WXG100 proteins are a group of proteins of approximately ∼100 residues in length that contain a conserved “Trp-Xaa-Gly (WXG)” motif. To investigate how specific sequence motifs translate into specific structural features, we determined the atomic structures of two representative complexes, the heterodimeric CFP-10/ESAT-6 complex and the homodimeric sagEsxA assembly. The overall structures of the two protein complexes are similar, with both forming a four-helix bundle, in which each monomer consists of a helix-loop-helix structural motif. However, the novelty of this contribution is that by using the iterative bio-informatics approach, we can show that the WXG100 protein superfamily can be divided into three subfamilies: CFP-10-, ESAT-6- and sagEsxA-like.

The sagEsxA-like proteins form a homodimer and the structure of the sagEsxA shows that the driving force for the interdimer interactions is principally hydrophobic in nature. At the inter-dimeric interface, hydrophobic residues are prevalent in sagEsxA-like proteins although there is a pair of hydrophilic residues Y18 and Q36 within the hydrophobic core of sagEsxA. The side chains of these residues form hydrogen bonds within the hydrophobic core of the four-helix-bundle complex (inset) and the presence of these hydrogen bond pairs between Y18 and Q36 is indicative of the anti-parallel homodimer arrangement found in the sagEsxA subfamily of WXG100 proteins. As a result, this conserved pair of mutations can be seen as a fingerprint of anti-parallel homodimeric WXG100 proteins. In addition, it contains a 310-helix with hydrogen bonds originating only from main chain atoms, whereas, the loop of sagEsxA (residues 43–48) consists only of a single tight β-turn. The CFP-10 subfamily is structurally more closely related to the sagEsxA than to the ESAT-6 subfamily. This is reflected by a root mean square deviation (r.m.s.d) of 2.07 Å for a superimposition of the core residues of CFP-10 (residues 11–83) and sagEsxA (residues 11–83), compared to an r.m.s.d. of 3.43 Å for the equivalent ESAT-6/sagEsxA superimposition. Secondly, by examining every WXG100 gene in its genetic context we could clearly show that all WXG100 genes from the Actinobacteria phylum are encoded in a bi-cistronic operon containing a CFP-10-like gene followed by an ESAT-6-like gene without exception, whereas, all the sagEsxA-like genes occur as mono-cistronic genes in the bacterial genomes belonging to Firmicutes. Interestingly, the sagEsxA FRET signal could only be detected after extensive heat treatment. This result shows that the homodimer is stable, and a FRET pair homodimer can only be reconstituted after heat dissociation.

>[2x]GAMSQIKLTPEELRSSAQKYTAGSQQVTEVLNLLTQEQAVIDENWDGSTFDSFEAQFNELSPKITEFAQLLEDINQQLLKVADIIEQTDADIASQISG>[2x]GSMKIDVVTIFPEYLQPVRQSLPGKAIDAGLVDVAVHDLRRWTHDVHKSVDDSPYGGGPGMVMKPTVWGDALDEICTSE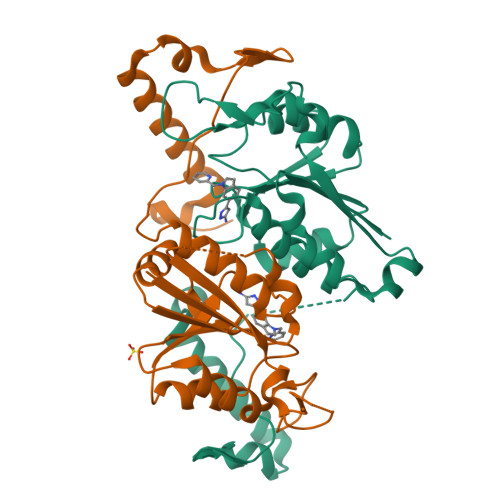TLLVVPTPAGYPFTQETAWQWSTEDHLVIACGRYEGIDQRVADDAATRMRVREVSIGDYVLNGGEAAALVIIEAVLRLVPGVLGNALSAQEDSHSEGMASLLEGPSYTRPPSWRGMDVPPVLLSGDHAKIAAWRAEQSRQRTIERRPDLLGFDSPTGEHGGDGLS>MKVGQDKVVTIRYTLQVEGEVLDQGELSYLHGHRNLIPGLEEALEGREEGEAFQAHVPAEKAYGATGHPGIIPPHATLDFQVEVVKVREATPEELLHGHAHPS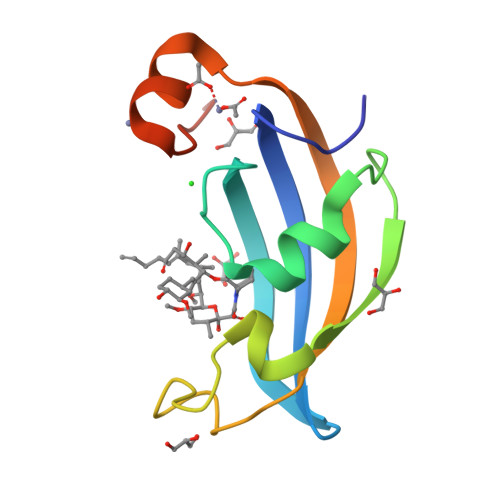GHHHHHH[2x]>[2x]MEFTVSTTEDLQRYRTECVSSLNIPADYVEKFKKWEFPEDDTTMCYIKCVFNKMQLFDDTEGPLVDNLVHQLAHGRDAEEVRTEVLKCVDKNTDNNACHWAFRGFKCFQKNNLSLIKASIKKD

Ae. aegypti OBP22 (AeOBP22) is a member of the OBP family of proteins that has been directly implicated in regulating these feeding behaviors. AeOBP22 is unusual in that it is expressed in multiple chemosensory tissues, including in the antenna, the proboscis of the females, the thoracic spiracles, in the male reproductive glands where it is transferred to the females during mating, and in the salivary glands. The monomeric forms of AeOBP22 are similar to other classical OBPs which consist of six α-helices stabilized by three disulfide bridges surrounding a hydrophobic pocket. Our results provide evidence that fatty acids are likely natural ligands for AeOBP22 and that the binding of long-chain fatty acids (C15-C20) is enhanced by a conformational change in the C-terminal tail that is critical to generate a high affinity binding site.

The third crystal form grows in the presence of cadmium and/or cobalt ions in the C121 space group and contains only monomers. Structures of the apo-state and the complexes formed with linoleic acid (C18:2) and AA (C20:4) were solved using cobalt SAD methods and refined to a resolution of 1.85 Å. In the bound state, AeOBP22 is unusual in that it contains a seventh C-terminal α-helix that forms one edge of the ligand-binding pocket. Small differences are seen in the position of helix-7, which rotates out slightly from the binding pocket in the presence of larger fatty acids such that the Cα at Ile120 is approximately 2 Å displaced from its position with shorter chain fatty acids. The NMR structure of the AeOBP22-AA complex superimposes with the crystal structure with an RMSD of 0.67 Å for the backbone atoms of residues 7–120 and confirms that the monomeric structure observed in the crystal is maintained in solution. The biggest differences between the structure are in the conformation of the loop between helices 4 and 5, which are involved in crystal packing, but which are dynamic in solution. The overall structure of the arachidonic acid ligand is similar to the structure observed in the crystal. However, even in the crystal there are differences in the ligand position in the two monomers in the asymmetric unit. However, the extent of unsaturation also impacts the affinity, with the more rigid AA (C20:4) having a lower affinity than the monounsaturated C20:1.> MHHHHHHSSGRENLYFQGKIDIHVLENFKN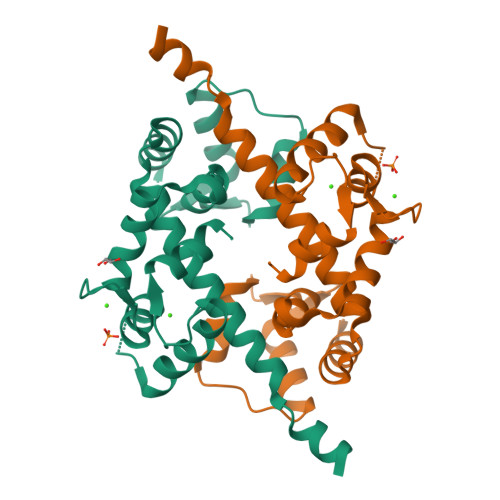YALMLRFQKLAMTIIAQQSNDYDVQKLKAAFLHLDEEGKGNITKLQLRKGLERSGLMLPPNFDLLLDQIDSDGSGNIDYTEFLAAAIDRRQLSKKLIYCAFRVFDVDNDGEITTAELAHVLFNGNKRGNITERDVNQVKKMIREVDKNGDGKIDFYEFSEMMKLTL methyl 6-[6-amino-2-(methylamino)-8-oxo-7,8-dihydro-1H-imidazo[4,5-g]quinazolin-4-yl]-5,6-dideoxy-3-O-methyl-beta-D-ribo-hexofuranoside 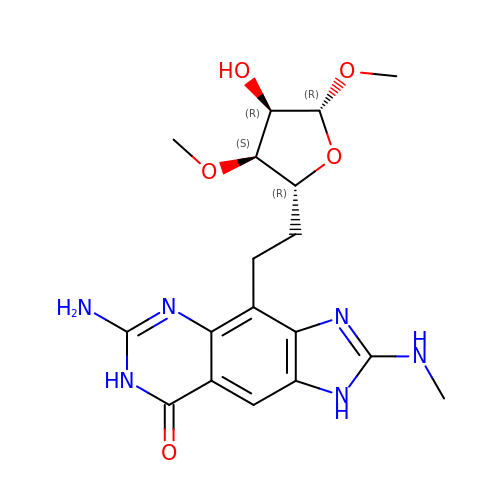| C18 H24 N6 O5 | AYNKUXIALNGELF-DSPGLSBSSA-N>MEIKDLKRLARYNPEKMAKIPVFQSERMLYDLYALLPGQAQKVHVHEGSDKVYYALEGEVVVRVGEEEALLAPG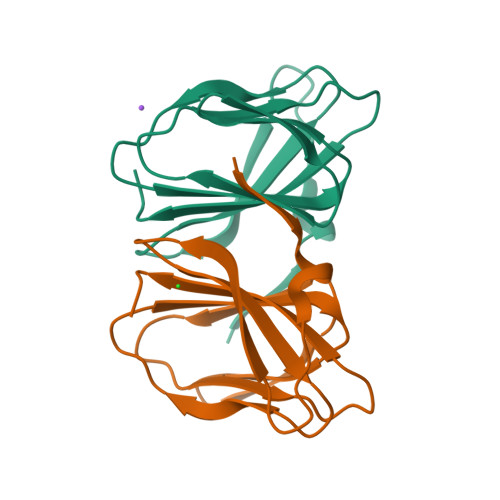MAAFAPAGAPHGVRNESASPALLLVVTAPRP[2x]>[2x]MAHHHHHHMDAVSETAKRAALDTSIKVDGRRLWDSLMEVAKIGATPKGGVCRLALTDLDKAARDLIVGWAKAAGCTVTVDTMGNVFMRRAGRVADAAPVVTGSHADSQPTGGRFDGIYGVLGGLEVIRSLNDHGIETEHPVEVVIWTNEEGSRFAPAMVASGVFAGVFPLEYG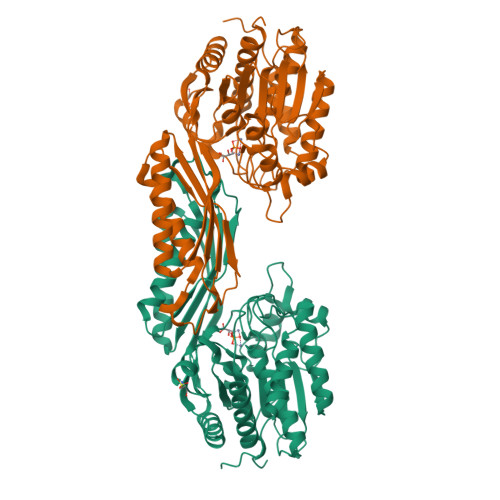LSRKDVDGKTIGEELARIGYAGDAPCGGRKLHAAFELHIEQGPILEAECKTIGVVTDAQGQRWYEITFTGQEAHAGPTPMPRRRDALLGASRVVDLVNRIGLDHAPYGCATVGMMQVHPNSRNVIPGRVFFTVDFRHPDDAVLAKMDAALRDGVARIAADIGLDTALEQIFYYAPIAFDSACVAAVRAAADRFGYSHRDIVSGAGHDACYLAQVAPTSMVFVPCIDGISHNEIEDATPAWIEAGANVLLHAMLSRACEPVS(2s,4R)-2-{4-[(2-chloro-4-fluorophenoxy)methyl]piperidine-1-carbonyl}-7-oxa-5-azaspiro[3.4]octan-6-one | C19 H22 Cl 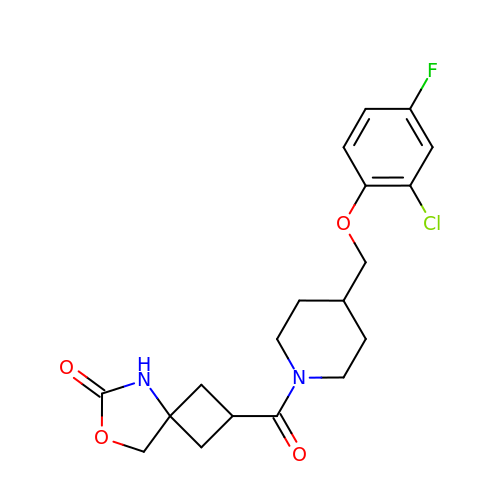F N2 O4 | ZXSYTHGPTJFVMM-XVDXERDNSA-N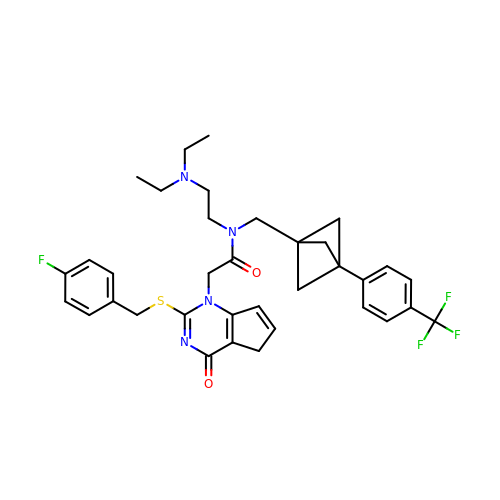~{N}-[2-(diethylamino)ethyl]-2-[2-[(4-fluorophenyl)methylsulfanyl]-4-oxidanylidene-5~{H}-cyclopenta[d]pyrimidin-1-yl]-~{N}-[[3-[4-(trifluoromethyl)phenyl]-1-bicyclo[1.1.1]pentanyl]methyl]ethanamide | C35 H38 F4 N4 O2 S | SHVFOCPBEIJQSO-AQOUDTPCSA-N> GPMDDKELIEYFKSQMKEDPDMASAVAAIRTLLEFLKRDKGETIQGLRANLTSAIETLCGVDSSVAVSSGGELFLRFISLASLEYSDYSKCKKIMIERGELFLRRISLSRNKIADLCHTFIKDGATILTHAYSRVVLRVLEAAVAAKKRFSVYVTESQPDLSGKKMAKALCHLNVPVTVVLDAAVGYIMEKADLVIVGAEGVVENG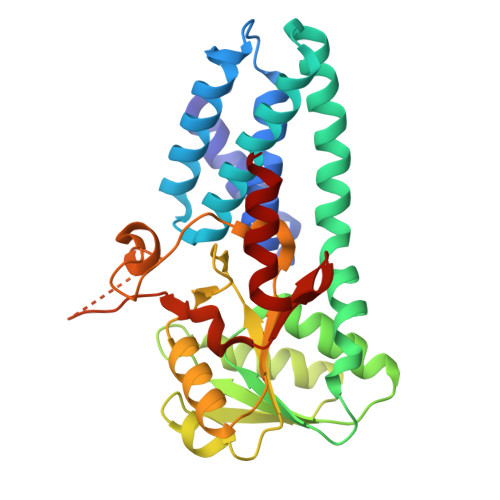GIINKIGTNQMAVCAKAQNKPFYVVAESFKFVRLFPLNQQDVPDKFKYKADTLKVAQTGQDLKEEHPWVDYTAPSLITLLFTDLGVLTPSAVSDELIKLYL> MLNPIVRKFQYGQHTVTLETGMMARQATAAVMVSMDDTAVFVTVVGQKKAKPGQDFFPLTVNYQERTYAAGRIPGSFFRREGRPSEGETLIARLIDRPIRPLFPEGFVNEVQVIATVVSVNPQVNPDIVAMIGASAALSLSGIPFNGPIGAARVGYINDQYVLNPTQDELKESKLDLVVAGTEAAVLMVESEAQLLSEDQMLGAVVFGHEQQQVVIQNINELVKEAGKPRWDWQPEPVNEALNARVAALAEARLSDAYRITDKQERYAQVDVIKSETIATLLAEDETLDENELGEILHAIEKNVVRSRVLAGEPRIDGREKDMIRGLDVRTGVLPRTHGSALFTRGETQALVTATLGTARDAQVLDELMGERTDTFLFHYNFPPYSVGETGMVGSPKRREIGH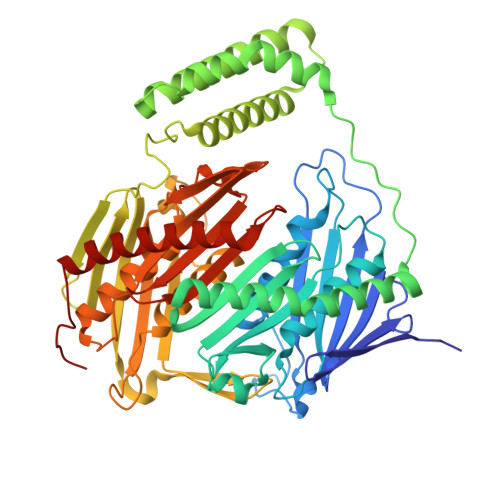GRLAKRGVLAVMPDMDKFPYTVRVVSEITESNGSSSMASVCGASLALMDAGVPIKAAVAGIAMGLVKEGDNYVVLSDILGDEDHLGDMDFKVAGSRDGISALQMDIKIEGITKEIMQVALNQAKGARLHILGVMEQAINAPRGDIS>[2x]KHSLPDLPYDYGALEPHINAQIMQLHHSKHHAAYVNNLNVTEEKYQEALAKGDVTAQ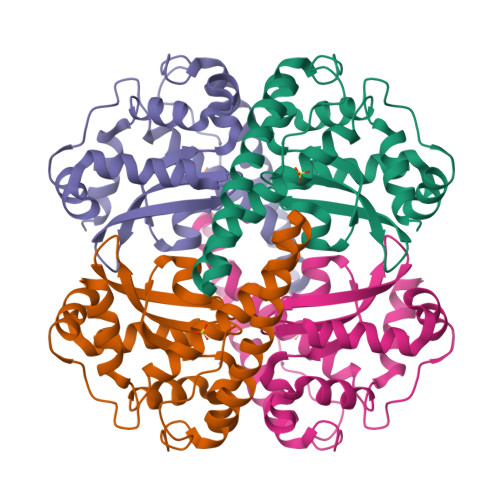IALQPALKFNGGGHINHSIFWTNLSPNGGGEPKGELLEAIKRDFGSFDKFKEKLTAASVGVQGSGWGWLGFNKERGHLQIAACPNADPLQGTTGLIPLLGIDVWEHAYYLQYKNVRPDYLKAIWNVINWENVTERYMACKK> MKDL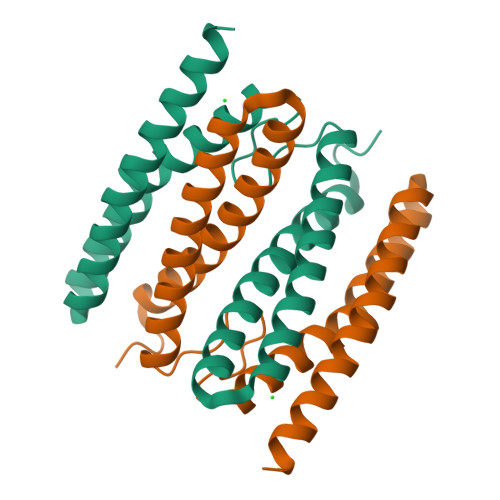KGTKTAENLKQGFIGESMANRRYLYFAKRADEEGYPEIAGLLRSIAEGETAHAFGHLDFIRQGGLTDPATDKPIGTLEQMIESAIAGETYEWTQMYPGFAKVAREEGFPEVAEWFETLARAEKSHAEKFQNVLKQLKGGT>MDTFVLDTSVFTNPDVYHQFEEDQLGAIENFISLASHTNANFFMPTSVYYEFTKMVSLGDLAPKFE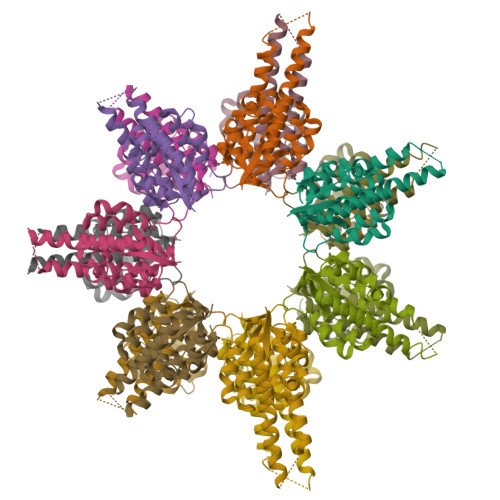LVVRIRSPRKWGLMVPAEFLYEFIEEVRYRINKGLRIAEEHTKEAGKLAEEEVGRVVNRLREKYREALRAGIIDSKEDVDVLLLSYELDAILVSGDEGLRKWADRVGIKLIDPKNLRYIMENLTKVGR[7x]>[4x]SNAMRKGS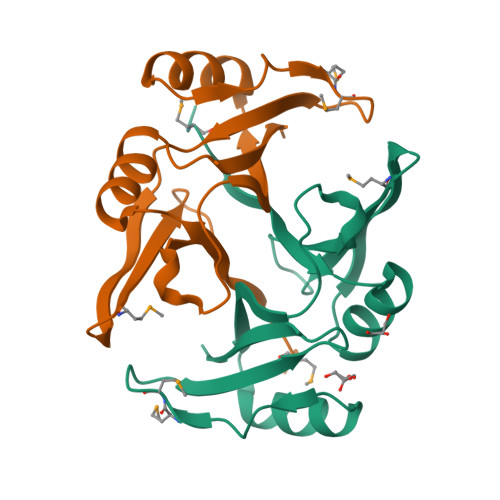LMIAYVHSATIIVSDQEKALDFYVNTLGFEKVFDNQLDPNMRFVTVVPPGAQTQVALGLPSWYEDGRKPGGYTGISLITRDIDEAYKTLTERGVTFTKPPEMMPWGQRATWFSDPDGNQFFLVEE> 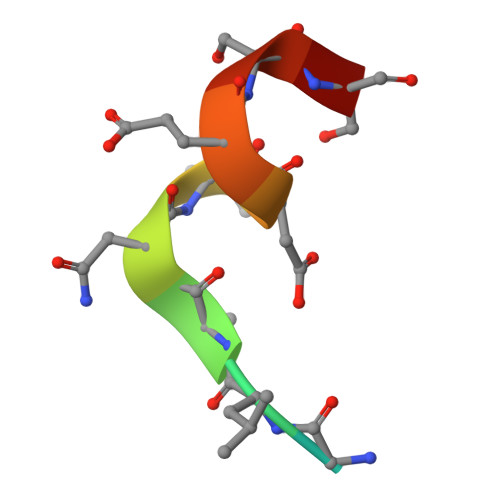GYGLANVDESSG> MATVTATTKVPEIRDVTRIERIGAHSHIRGLGLDDALEPRQASQGMVGQLAARRAAGVVLEMIREGKIAGRAVLIAGQPGTGKTAIAMGMAQALGPDTPFTAIAGSEIFSLEMSKTEALTQAFRRSIGVRIKEETEIIEGEVVEIQIDRPATGTGSKVGKLTLKTTEMETIYDLGTKMIESLTKDKVQAGDVITIDKATGKISKLGRSFTRARDYDAMGSQTKFVQCPDGELQKRKEVVHTVSLHEIDVINSRTQGFLALFSGDTGEIKSEVREQINAKVAEWREEGKAEIIPGVLFIDEVHMLDIESFSFLNRALESDMAPVLIMATNRGITRIRGTSYQSPHGIPIDLLDRLLIVSTTPYSEKDTKQILRIRCEEEDVEMSEDAYTVLTRIGLETSLRYAIQLITAASLVCRKRKGTEVQVDDIKRV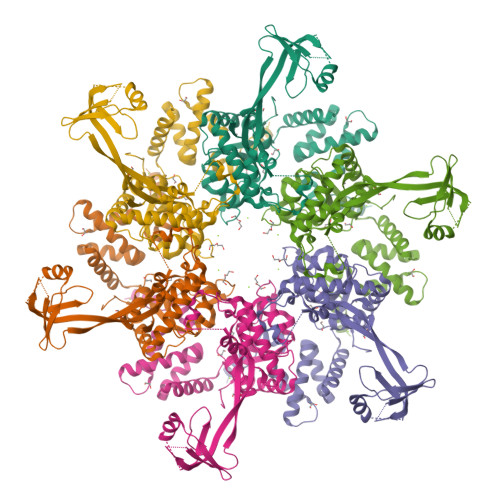YSLFLDESRSTQYMKEYQDAFLFNELKGETMDTS> GGVRGSLGSPGNRENKEKKVFISLVGSRGLGCSISSGPIQKPGIFISHVKPGSLSAEVGLEIGDQIVEVNGVDFSNLDHKEAVNVLKSSRSLTISIVAAAGRE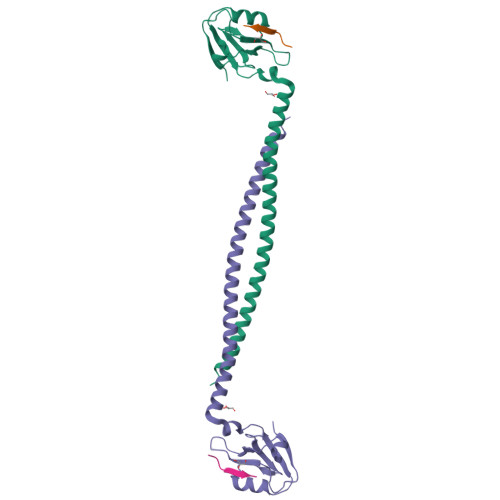LFMTDRERLAEARQRELQRQELLMQKRLAMESNKILQEQQEMERQRRKEIAQKAAEENERYRKEMEQIVEEEEKF;> QQKKNLSFTNPGLDTTDL> TRFTEEYQLFEELGKGAFSVVRRCVKVLAGQEYAAKIINTKKLSARDHQKLEREARICRLLKHPNIVRLHDSISEEGHHYLIFDLVTGGELFEDIVAREYYSEADASHCIQQILEAVLHCHQMGVVHRNLKPENLLLASKLKGAAVKLADFGLAIEVEGEQQAWFGFAGTPGYLSPEVLRKDPYGKPVDLWA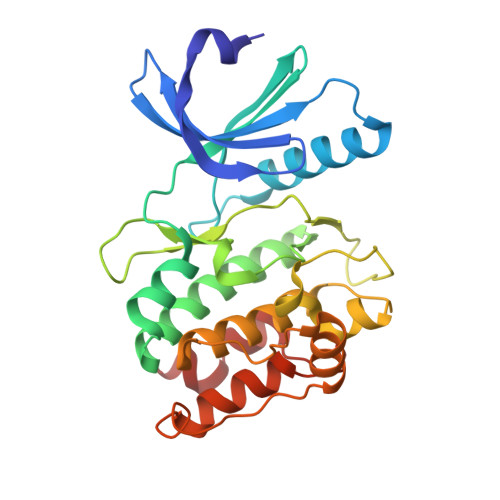CGVILYILLVGYPPFWDEDQHRLYKQIKAGAYDFPSPEWDTVTPEAKDLINKMLTINPSKRITAAEALKHPWISHR> ELICIVQRVNESFSLHSGFGGNVYSMKTEPMTGFTNVTKGASVINQKDWIGFGDARTDLTNDQFPASSDVPLAVAKKFRSLSGASLMLSAFGPPGKVDYLYQGCGKEKVFYEGVNWSPEAGIDCFGSNWTQTKKDFYSRIYEAARSSTCMTLVNSLDTKISSTTATAGTASSCSSSWMKSPLWYAESSVNPGAKPQVCGTEQSATFTLPTSFGIYKCNKHVVQLCYFVYENKAKFNTFGCGDYYQNYYDGNGNLIGGMDNRVAAYRGIANAGVKIECPSKILNPGTYSIKSTPRFLLVPKRSYCFDTDGG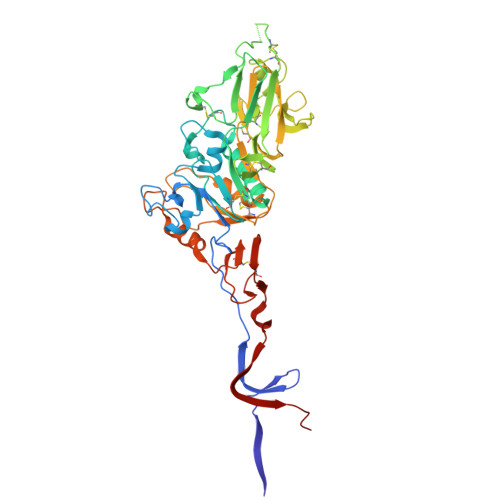YPIQVVQSEWSASRRSDNATEEACLQTEGCIFIKKTTPYVGEAADNAGDIEMRQLLSGLGNNDTVCVSQSGYTKGETPFVKDYLSPPKYGRCQLKTDSGRIPTLPSGLIIPQAGTDS1-(4-acetyl-6-pyridin-3-yl-1H-benzimidazol-2-yl)-3-ethylurea 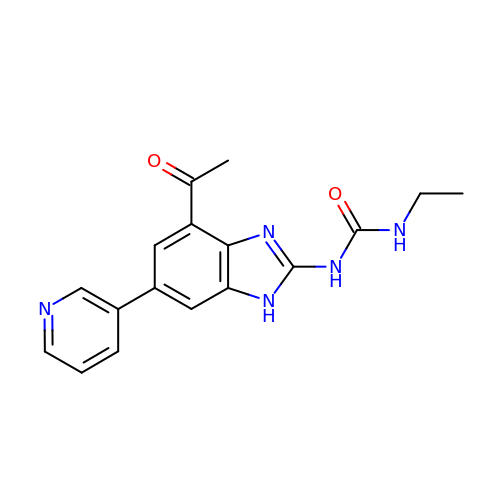| C17 H17 N5 O2 | KDHATIBQZJAMKQ-UHFFFAOYSA-N> GPGSEFRQDKMREEGLQLVSMIR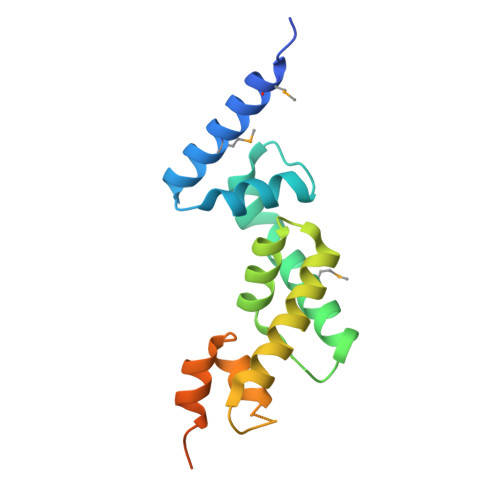EGEAAGACPEEIFSALQYSGTEVPLQWLRSELPYVLEMVAELAGQQDPGLGAFSCQEARRAWLDRHGNLDEAVEECVRTRRRKVQELQSLGFGPEEGSLQALFQHGGDVSRALTELQRQRLEPFRQRLWDSGPEPTPSWDGPD(2R,3S,4R,5S,6R)-2-(hydroxymethyl)-6-[(E)-3-quinolin-6-ylprop-2-enyl]oxane-3,4,5-triol 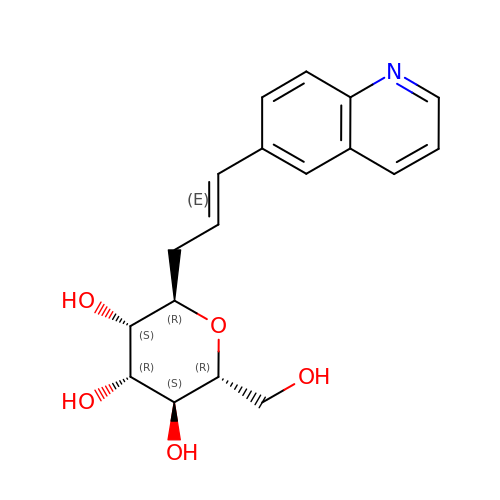| C18 H21 N O5 | SJKMSFJIONHVCI-GBPXCZALSA-N> MACPISQSVSQPVDERLTRAAIFLVVTINPGKAAEVAVRTLCGTLSSLVRGVGFRILDGGLSCVMGVSSGGWERLFGDEKPEYLHVFQEINGVHHAPSTPGDLLFHIRAARMDLCFELASRILSDLGSSVCVVDSVQGFRYFDDRDLLGFVDGTENPVAQAAVDATLIGEEDHTFS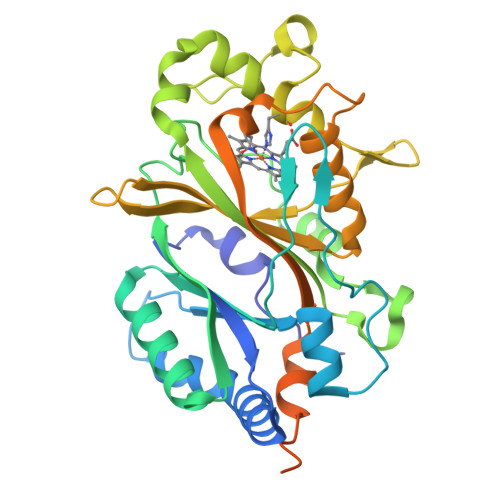GGSYVIVQKYLHDLDKWNAIPVEQQEKIIGREKLSDIELKDADKPSYAHNVLTSIEEDGEDVDILRDNMPFGDPGKGEFGTYFIGYSRKPARIERMLENMFVGNPPGNYDRILDVSRAITGTLFFIPTVSFLDSVEPQPSVSQQTDDAKYIYDSPGTKGESGSLNIGSLKKEVQDEENLYFQGGSGGHHHHHHH> CYIQNCPL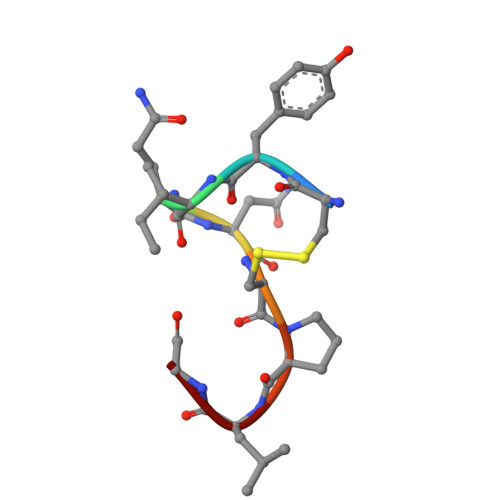G> LPTSNPAQELEARQLGRTTRDDLINGNSASCRDVIFIYARGSTETGNLGTLGPSIASNLESAFGKDGVWIQG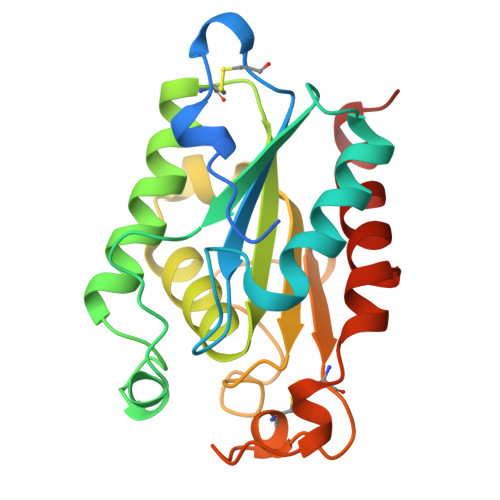VGGAYRATLGDLALPRGTSSAAIREMLGLFQQANTKCPDATLIAGGYSQGAALAAASIEDLDSAIRDKIAGTVLFGYTKNLQNRGRIPNYPADRTKVFCNTGDLVCTGSLIVAAPHLAYGPDARGPAPEFLIEKVRAVRGSA>ESNQQIADFDKEKATLDEADIDERMKLAQAFNDSLNNVVSGDPWSEEMKKKGRAEYARMLEIHERMGHVEIPVIDVDLPVYAGTAEEVLQQGAGHLEGTSLPIGGNSTHAVITAHTGLPTAKMFTDLTKLKVGDKFYVHNIKEVMAYQVDQVKVIEPTNFDDLLIVPGHDYVTLLTCTPYMINTHRLLVRGHRIPYVAEV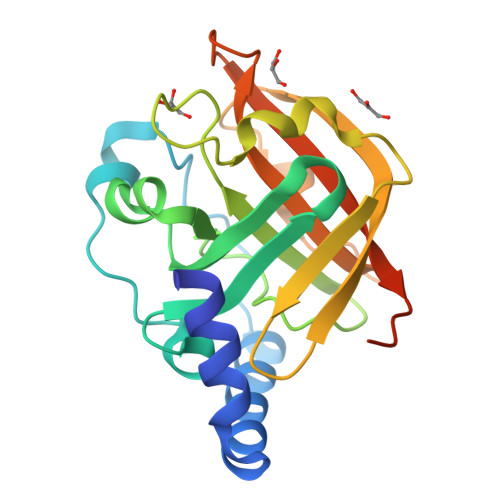EEEFIAANKLSH[2x]One highly versatile encapsulation system has been engineered from the capsid-forming enzyme lumazine synthase from the hyperthermophilic bacterium Aquifex aeolicus. In nature, these structures encapsulate riboflavin synthase, an enzyme that converts lumazine to riboflavin. In the structures of the AaLS variants, the pentamer is the common and exclusive building block for all assemblies. Here, we elucidate the structures of the AaLS protein containers by native mass spectrometry (MS) and cryo-EM single-particle reconstruction techniques.

The best variant, AaLS-13, possesses seven additional mutations that further increase the container's net negative charge and enhance its ability to bind positively charged proteins both in vivo and in vitro. The 3D classification, followed by refinement using 9,900 particles, resulted in an EM map resolved to 5.2 Å resolution. Like its evolutionary parent, AaLS-13 has a highly porous cage structure constructed exclusively from pentameric building blocks, but, in contrast to AaLS-neg, it adopts icosahedral symmetry. The 39-nm wide, ∼6-MDa large sphere is assembled from 72 pentamers (360 subunits), twice as many as AaLS-neg. Its internal volume (15,600 nm3) is 3.7 times larger than that of AaLS-neg (4,200 nm3) and 58 times larger than that of AaLS-wt (270 nm3), accounting for its enhanced loading capacity. The AaLS-13 cage architecture can be best viewed as an extended dodecahedron, the dual counterpart of an icosahedron, with each face consisting of a central pentamer surrounded by five others (12 × 30-mer). In contrast, the AaLS-13 assembly is not skewed, and its porous surface avoids offending contacts that could arise when a pentamer is packed inside a pseudohexagonal hole. The A118D mutation, in particular, induces a substantial displacement of the α4 helix to avoid steric and electrostatic clashes. A remarkable feature of the negatively supercharged AaLS assemblies is that roughly 30% of the protomers (48/180 for AaLS-neg and 120/360 for AaLS-13) lack inter-pentamer interactions, leaving large pores in the shell wall.

>[360x]MEIYEGKLTAEGLRFGIVASRFNHALVGRLVEGAIDCIVRHGGREEDITLVCVPGSWEIPVAAGELARKEDIDAVIAIGVLIEGAEPHFDYIASEVSKGLANLSLELRKPISFGDITDDELEEAIECAGTEHGNKGWEAALSAIEMANLFKSLRLEHHHHH> MSLLNNKAGVISRLADFLGFRPKTGDIDVMNRQSVGSVTISQLAKGFYEPNIESAINDVHNFSIKDVGTIITNKTGVSPEGVSQTDYWAFSGTVTDDSLPPGSPITVLVFGLPVSATTGMTAIEFVAKVRVALQEAIASFTAIN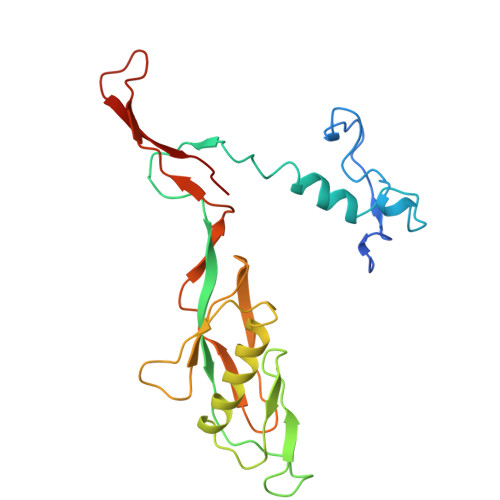SYKDHPTDGSKLEVTYLDNQKHVLSTYSTYGITISQEIISESKPGYGTWNLLGAQTVTLDNQQTPTVFYHFERTA>[2x]MSKTFAEIAEAFLEPEAVRIAKEAVEEYGDHERKIIQIGIHFQVCCMFCDEYLSTNGSDRFVLIEGRKRGTAVSLQNELCKSYDLEPLPFLCDIFDREEKQFVEIGITRKADDSYFQSKFGKLGNSCKIFVFSYDGRLDKNCEGPMEEQKLRIFSFLATAADFLRKENMFNEIFLPDNEETIIEMKKGKTFLELRDESVPLPFQTYEQMKDYCEKFKGNPRELASKVSQMQSNIKLPIKHYEQNKFRQIRLPKGPMAPYTHKFLMEEAWMFTKISDPERSRAGEILIDFFKKGNLSAIRPKDKPLQGKYPIHYKNLWNQIKAAIADRTMVINENDHSEFLGGIGRASKKIPEISLTQDVITTEGLKQSENKLPEPRSFPRWFNAEWMWAIKDSDLTGWVPMAEYPPADNELEDYAEHLNKTMEGVLQGTNCAREMGKCILTVGALMTECRLFPGKIKVVPIYARSKERKSMQEGLPVPSEMDCLFGICVKSKSHLNKDDGMYTIITFEFSIREPNLEKHQKYTVFEAGHTTVRMKKGESVIGREVPLYLYCRTTALSKIKNDWLSKARRCFITTMDTVETICLRESAKAEENLVEKTLNEKQMWIGKKNGELIAQPLREALRVQLVQQFYFCIYNDSQLEGFCNEQKKILMALEGDKKNKSSFGFNPEGLLEKIEECLINNPMCLFMAQRLNELVIEASKRGAKFFKTD;>MEINPYLMFLNNDVTSLISTTYPYTGPPPMSHGSSTKYTLETIKRTYDYSRTSVEKTSKVFNIPRRKFCNCLEDKDELVKPTGNVDISSLLGLAEMMEKRMGEGFFKHCVMEAETEILKMHFSRLTEGRQTYDWTSERNMPAATALQLTVDAIKETEGPFKGTTMLEYCNKMIEMLDWKEIKFKKVKTVVRREKDKRSGKEIKTKVPVMGIDSIKHDEFLIRALTINTMAKDGERGKLQRRAIATPGMIVRPFSKIVETVAQKICEKLKESGLPVGGNEKKAKLKTTVTSLNARMNSDQFAVNITGDNSKWNECQQPEAYLALLAYITKDSSDLMKDLCSVAPVLFCNKFVKLGQGIRLSNKRKTKEVIIKAEKMGKYKNLMREEYKNLFEPLEKYIQKDVCFLPGGMLMGMFNMLSTVLGVSTLCYMDEELKAKGCFWTGLQSSDDFVLFAVASNWSNIHWTIRRFNAVCKLIGINMSLEKSYGSLPELFEFTSMFFDGEFVSNLAMELPAFTTAG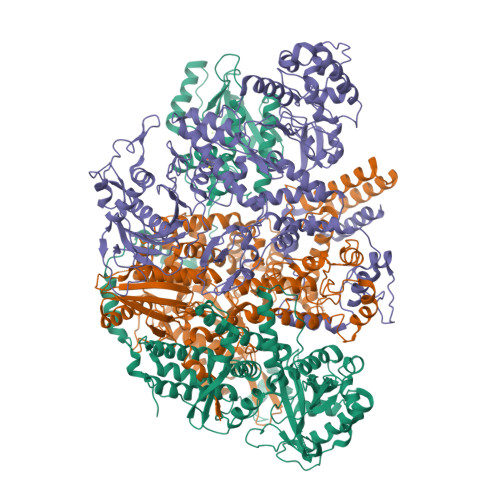VNEGVDFTAAMSIIKTNMINNSLSPSTALMALRICLQEFRATYRVHPWDSRVKGGRMKIINEFIKTIENKDGLLIADGGKLMNNISTLHIPEEVLKFEKMDEQYRNRVFNPKNPFTNFDKTIDIFRAHGPIRVEENEAVVSTHSFRTRANRTLLNTDMRAMMAEEKRYQMVCDMFKSVFESADINPPIGAMSIGEAIEEKLLERAKMKRDIGAIEDSEYEEIKDIIRDAKKARLESR[2x];>[2x]MSLLLTIAKEYKRLCQDAKAAQMMTVGTVSNYTTFKKWTTSRKEKNPSLRMRWAMSSKFPIIANKRMLEEAQIPKEHNNVALWEDTEDVSKRDHVLASASCINYWNFCGPCVNNSEVIKEVYKSRFGRLERRKEIMWKELRFTLVDRQRRRVDTQPVEQRLRTGEIKDLQMWTLFEDEAPLASKFILDNYGLVKEMRSKFANKPLNKEVVAHMLEKQFNPESRFLPVFGAIRPERMELIHALGGETWIQEANTAGISNVDQRKNDIRAVCRKVCLAANASIMNAKSKLVEYIKSTSMRIGETERKLEELILETDDVSPEVTLCKSALGGQLGKTLSFGPMLLKKISGSGVKVKDTVYIQGVRAVQFEYWSEQEEFYGEYKSATALFSRKERSLEWITIGGGINEDRKRLLAMCMIFCRDGDYFKDAPATITMADLSTKLGREIPYQYVMMNWIQKSEDNLEALLYSRGIVETNPGKMGSSMGIDGSKRAIKSLRAVTIQSGKIDMPESKEKIHLELSDNLEAFDSSGRIVATILDLPSDKKVTFQDVSFQHPDLAVLRDEKTAITKGYEALIKRLGTGDNDIPSLIAKKDYLSLYNLPEVKLMAPLIRPNRKGVYSRVARKLVSTQVTTGHYSLHELIKVLPFTYFAPKQGMFEGRLFFSNDSFVEPGVNNNVFSWSKADSSKIYCHGIAIRVPLVVGDEHMDTSLALLEGFSVCENDPRAPMVTRQDLIDVGFGQKVRLFVGQGSVRTFKRTASQRAASSDVNKNVKKIKMSNARENLYFQ>MNDFHRDTWAEVDLDAIYDNVENLRRLLPDDTHIMAVVKANAYGHGDVQVARTALEAGASRLAVAFLDEALALREKGIEAPILVLGASRPADAALAAQQRIALTVFRSDWLEEASALYSGPFPIHFHLKMDTGMGRLGVKDEEETKRIVALIERHPHFVLEGLYTHFATADEVNTDYFSYQYTRFLHMLEWLPSRPPLVHCANSAASLRFPDRTFNMVRFGIAMYGLAPSPGIKPLLPYPLKEAFSLHSRLVHVKKLQPGEKVSYGATYTAQTEEWIGTIPIGYADGWLRRLQHFHVLVDGQKAPIVGRICMDQCMIRLPGPL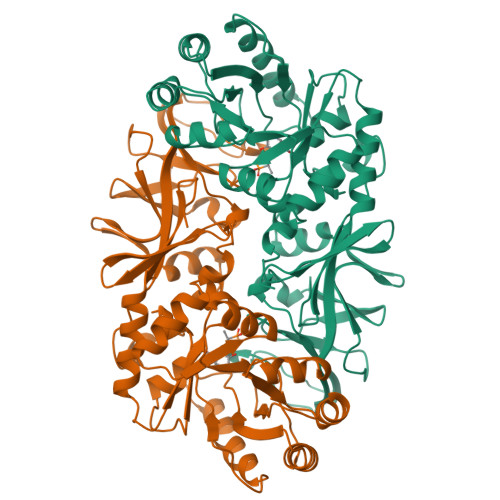PVGTKVTLIGRQGDEVISIDDVARHLETINYEVPCTISYRVPRIFFRHKRIMEVRNAIGAGESSA[2x]>GSHMNLF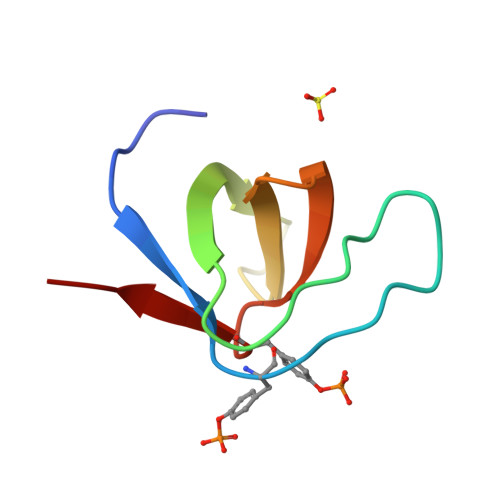VALYDFVASGDNTLSITKGEKLRVLGYNQNGEWSEVRSKNGQGWVPSNYITPVN[2x]> G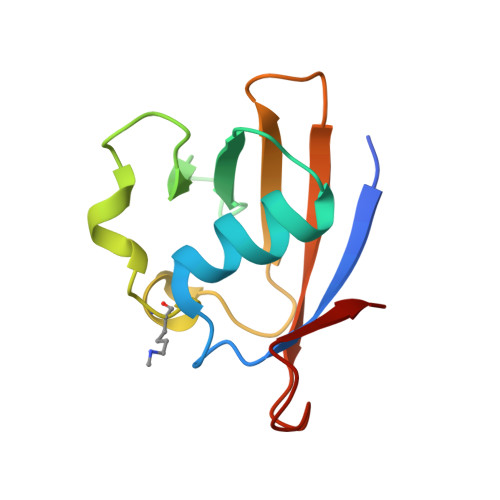SHSKPEVTVRLNVHKVTVLTLQDKIVKEKFAMVAPDVQIEDGKGTILISSEEGETEANNHKKLSEFGIRNGSRLQADDFLQDYTLLINILHSEDLGKDVEFEVV>MTSIIKIDLESKTPIYKQIADQIIELIAKGELKPGDKLPSIRELASMLGVNMLTVNKAYNYLVDEGFIVVQKRRYVVKSEVRDESWRNMLRVIIYRALASNMSKDEIVNEINRVVSEVNSK[2x]

The thermoacidophilic model crenarchaeote Sulfolobus acidocaldarius is predicted to harbor a gene encoding a putative GntR-type TF belonging to the YtrA subfamily. Closer inspection of the amino acid sequence encoded by the concerned gene (Saci_1851) learned that the C-terminal E-O domain of this 121-amino acid protein consists of about 50 amino acids predicted to fold into two α-helices, thus classifying it as a member of the YtrA subfamily. YtrASa performs an (auto-)repression function by interacting with high specificity and affinity with a 32-bp long inverted repeat. YtrASa represses the transcription of an operon encoding its own gene and a membrane protein and of a second gene encoding a membrane protein by interacting with a binding site that fully covers the transcription initiation site.

A crystallographic analysis of YtrASa yielded a structure at 3.0 Å resolution. The 14-kDa YtrASa protein crystallized as a dimer with the asymmetric unit of the crystal structure containing a homodimer with an exclusive α-helical structure. Each monomeric unit displays an N-terminal DNA-binding domain harboring the typical GntR-like wHTH motif (α1–α3) and a short C-terminal E-O domain, consisting of two α helices (α4–α5) that mediate dimerization, which is a typical feature for YtrA-like regulators. Upon comparing the YtrASa structure with that of the only described bacterial YtrA-type crystal structure, CGL2947 of C. glutamicum, major structural differences are observed despite the similar topological organization. The distance between the two monomeric Arg42 residues, located in wHTH domain, amounts 36 Å, which is similar to the length of one turn of the DNA helix. This is only about half of the distance between corresponding monomeric residues in the C. glutamicum YtrA structure. For one of the YtrASa chains, the α5 helix could not be modeled due to poor electron density, likely explained by a flexible behavior of these C-terminal helices within the crystal. Furthermore, the alignment of individual monomeric chains from within the same dimer demonstrated that the E-O domain has an asymmetric nature. Although these observations might be ascribed to the crystal packing and are not necessarily biologically relevant, the short length of α4 underlies a compact E-O domain regardless of its exact conformation and a shorter distance between the two monomeric DNA-binding domains in comparison to other YtrA-like regulators.> MRTFFVGGNWKANPKTVEEAEKLIEMLNGAKVEGNVEVVVAAPFIFLPTLQQKLRKDWKVSAENVFTKPNGAFTGEVTVPMIKSFGIEWTILGHSERRDILKEDDEFLAAKAKFALENGMKIIYCCGEHLSEREAGKASEFVSAQIEKMIPAIPAGKWDDVVIAYEPIWAIGTGKVASTQDAQEMCKVIRDILAAKVGADIANKVRILYGGSVKP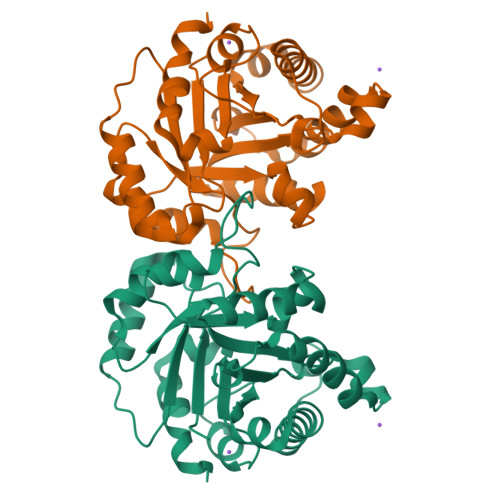NNCNELAACPDVDGFLVGGASLEPGFINIVNSNVHSK ATP-sensitive potassium channels (KATP) are ion channels that selectively allow potassium ions to permeate the cell. Specifically, they are inhibited by ATP and activated by Mg-ADP. Previous studies have established that the functional KATP channel is a hetero-octamer composed of four inward-rectifying potassium channel 6 (Kir6) subunits and four sulfonylurea receptor (SUR) regulatory subunits. KATP channels in pancreatic islets are composed of Kir6.2 channel subunits and SUR1 regulatory subunits.

The second structure is the KATP channel in complex with ATPγS alone, which is solved to 4.4 Å resolution (abbreviated, ATP state). Therefore, we applied ATPγS, a slowly hydrolyzable and functional ATP analog, to stabilize the structures of the KATP channel with and without GBM. The overall KATP channel structure and SUR1 conformation in the ATP + GBM state is almost identical to that in the ATP state based on our density maps. In the ATP and ATP + GBM state structures, SUR1 is in an inward-facing conformation. We observed ATP density only in the NBD1 degenerate site but not in the NBD2 consensus site, which suggests that the degenerate site has a higher affinity for Mg-free ATP, and ATP alone is not able to drive the dimerization of SUR1 NBDs. Here, we refer to class 1 structure as the “T state” (the tense state) and class 2 as the “R state” (the relaxed state). Instead, they possibly reflect the endogenous mobility of the CTDs in the Kir6.2-inhibited state, because we observed similar conformational heterogeneity of the KATP channel in the ATP state and the Mg-ADP state as described later.

>MLSRKGIIPEEYVLTRLAEDPAEPRYRTRERRARFVSKKGNCNVAHKNIREQGRFLQDVFTTLVDLKWPHTLLIFTMSFLCSWLLFAMVWWLIAFAHGDLAPGEGTNVPCVTSIHSFSSAFLFSIEVQVTIGFGGRMVTEECPLAILILIVQNIVGLMINAIMLGCIFMKTAQAHRRAETLIFSKHAVITLRHGRLCFMLRVGDLRKSMIISATIHMQVVRKTTSPEGEVVPLHQVDIPMENGVGGNGIFLVAPLIIYHVIDSNSPLYDLAPSDLHHHQDLEIIVILEGVVETTGITTQARTSYLADEILWGQRFVPIVAEEDGRYSVDYSKFGNTIKVPTPLCTARQLDEDRSLLDALTLASSRGPLRKRSVAVAKAKPKFSISPDSLS[4x];>[4x]MPLAFCGTENHSAAYRVDQGVLNNGCFVDALNVVPHVFLLFITFPILFIGWGSQSSKVHIHHSTWLHFPGHNLRWILTFILLFVLVCEIAEGILSDGVTESRHLHLYMPAGMAFMAAITSVVYYHNIETSNFPKLLIALLIYWTLAFITKTIKFVKFYDHAIGFSQLRFCLTGLLVILYGMLLLVEVNVIRVRRYIFFKTPREVKPPEDLQDLGVRFLQPFVNLLSKGTYWWMNAFIKTAHKKPIDLRAIGKLPIAMRALTNYQRLCVAFDAQARKDTQSPQGARAIWRALCHAFGRRLILSSTFRILADLLGFAGPLCIFGIVDHLGKENHVFQPKTQFLGVYFVSSQEFLGNAYVLAVLLFLALLLQRTFLQASYYVAIETGINLRGAIQTKIYNKIMHLSTSNLSMGEMTAGQICNLVAIDTNQLMWFFFLCPNLWAMPVQIIVGVILLYYILGVSALIGAAVIILLAPVQYFVATKLSQAQRSTLEHSNERLKQTNEMLRGMKLLKLYAWESIFCSRVEVTRRKEMTSLRAFAVYTSISIFMNTAIPIAAVLITFVGHVSFFKESDLSPSVAFASLSLFHILVTPLFLLSSVVRSTVKALVSVQKLSEFLSSAEIREEQCAPREPAPQGQAGKYQAVPLKVVNRKRPAREEVRDLLGPLQRLAPSMDGDADNFCVQIIGGFFTWTPDGIPTLSNITIRIPRGQLTMIVGQVGCGKSSLLLATLGEMQKVSGAVFWNSNLPDSEGEDPSSPERETAAGSDIRSRGPVAYASQKPWLLNATVEENITFESPFNKQRYKMVIEACSLQPDIDILPHGDQTQIGERGINLSGGQRQRISVARALYQQTNVVFLDDPFSALDVHLSDHLMQAGILELLRDDKRTVVLVTHKLQYLPHADWIIAMKDGTIQREGTLKDFQRSECQLFEHWKTLMNRQDQELEKETVMERKASEPSQGLPRAMSSRDGLLLDEEEEEEEAAESEEDDNLSSVLHQRAKIPWRACTKYLSSAGILLLSLLVFSQLLKHMVLVAIDYWLAKWTDSALVLSPAARNCSLSQECDLDQSVYAMVFTLLCSLGIVLCLVTSVTVEWTGLKVAKRLHRSLLNRIILAPMRFFETTPLGSILNRFSSDCNTIDQHIPSTLECLSRSTLLCVSALTVISYVTPVFLVALLPLAVVCYFIQKYFRVASRDLQQLDDTTQLPLLSHFAETVEGLTTIRAFRYEARFQQKLLEYTDSNNIASLFLTAANRWLEVRMEYIGACVVLIAAATSISNSLHRELSAGLVGLGLTYALMVSNYLNWMVRNLADMEIQLGAVKRIHALLKTEAESYEGLLAPSLIPKNWPDQGKIQIQNLSVRYDSSLKPVLKHVNALISPGQKIGICGRTGSGKSSFSLAFFRMVDMFEGRIIIDGIDIAKLPLHTLRSRLSIILQDPVLFSGTIRFNLDPEKKCSDSTLWEALEIAQLKLVVKALPGGLDAIITEGGENFSQGQRQLFCLARAFVRKTSIFIMDEATASIDMATENILQKVVMTAFADRTVVTIAHRVHTILSADLVMVLKRGAILEFDKPETLLSQKDSVFASFVRADK>[2x]MYRTAASRARALKGVLTRSLRPARYASSSAVAETSSSTPAYLSWLSGGSRAALTSLDMPLQGVSLPPPLADKVEPSKLQITTLPNGLKIASETTPNPAASIGLYVDCG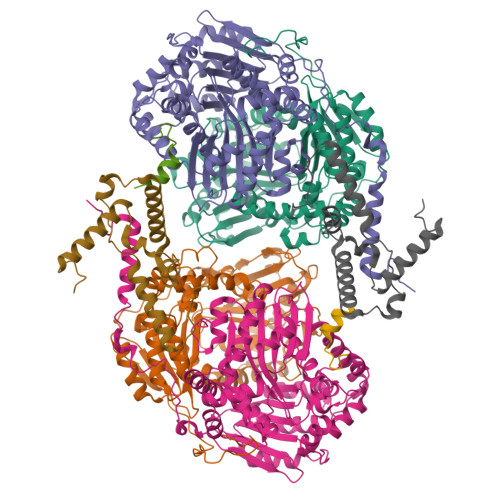SIYEAPYFHGATHLLERMAFKSTLNRTHFRLVREIEAIGGNTSASASREQMSYTIDALKTYVPEMVEVLIDSVRNPAFLDWEVNEELRKMKVEIAELAKNPMGFLLEAIHSAGYSGPLASPLYAPESALDRLNGELLEEFMTENFTAARMVLAASGVEHEELLKVAEPLTSDLPNVPPQLAPKSQYVGGDFRQHTGGEATHFAVAFEVPGWNNEKEAVTATVLQMLMGGGGSFSAGGPGKGMHSWLYRRVLNEYQEVQSCTAFTSIFNDTGLFGIYGCSSPQFAAKAIELAAKELKDVAGGKVNQAHLDRAKAATKSAVLMNLESRMIAAEDIGRQILTYGERKPVDQFLKSVDQLTLKDIADFTSKVISKPLTMGSFGDVLAVPSYDTISSKFR;>[2x]MAMKNLLSLARRSQRRLFLTQATRSSSSFSAIDSVPASASPTALSPPPPHLMPYDHAAEIIKNKIKKLENPDKRFLKYASPHPILASHNHILSAPETRVTTLPNGLRVATESNLSAKTATVGVWIDAGSRFESDETNGTAHFLEHMIFKGTDRRTVRALEEEIEDIGGHLNAYTSREQTTYYAKVLDSNVNQALDVLADILQNSKFEEQRINRERDVILREMQEVEGQTDEVVLDHLHATAFQYTPLGRTILGPAQNVKSITREDLQNYIKTHYTASRMVIAAAGAVKHEEVVEQVKKLFTKLSSDPTTTSQLVANEPASFTGSEVRMIDDDLPLAQFAVAFEGASWTDPDSVALMVMQTMLGSWNKNVGGGKHVGSDLTQRVAINEIAESIMAFNTNYKDTGLFGVYAVAKADCLDDLSYAIMYEVTKLAYRVSDADVTRARNQLKSSLLLHMDGTSPIAEDIGRQLLTYGRRIPTAELFARIDAVDASTVKRVANKYIYDKDIAISAIGPIQDLPDYNKFRRRTYWNRY;>[2x]MLRVAGRRLFSVSQRSSTATSFVVSRDHTLSDGGGDSSSAPRSLPSADLSSYHRSLIRGFSSQVLAQGNEIGFGSEVPATVEAVKTPNSKIVYDDHNHERYPPGDPSKRAFAYFVLSGGRFVYASVLRLLVLKLIVSMSASKDVLALASLEVDLGSIEPGTTVTVKWRGKPVFIRRRTEDDIKLANSVDVGSLRDPQEDSVRVKNPEWLVVVGVCTHLGCIPLPNAGDYGGWFCPCHGSHYDISGRIRKGPAPYNLEVPTYSFLEENKLLIG;>MASFLQRLVDPRKNFLARMHMKSVSNRLRRYGLRYDDLYDPLYDLDIKEALNRLPREIVDARNQRLMRAMDLSMKHEYLPDNLQAVQTPFRSYLQDMLALVKRERAEREALGALPLYQRTIP[2x]Bestrophin-1 (Best1) and bestrophin-2 (Best2) are two members of the bestrophin family of calcium (Ca2+)-activated chloride (Cl−) channels with critical involvement in ocular physiology and direct pathological relevance. The bestrophins are a family of Ca2+-activated anion channels consisting of four members (Best1–4) in mammals. The overall architecture of hBest1 and hBest2 resembles the pentameric assembly previously shown by KpBest, cBest1 and bBest2, and retains the two landmark permeation constrictions, the neck and aperture, in the ion conducting pathway. Ample electrophysiological evidence indicates that the neck and aperture serve as dual Ca2+-dependent channel “gates”, as disrupting either of them partially impairs Ca2+-dependence while disrupting both makes the channel completely Ca2+-independent.

To elucidate the architecture of human bestrophins, we purified WT hBest1 and hBest2 for single-particle cryo-EM analysis in the absence of Ca2+ (EGTA), or after a 30 s spike of 1 μM or 5 mM Ca2+. Under both 1 μM and 5 mM Ca2+ conditions, most of the hBest1/hBest2 particles (~90–95%) were in a Ca2+-bound closed state, which is very similar to the Ca2+-unbound closed state. In both hBest1 and hBest2 structures, the neck is formed by the same set of hydrophobic residues (I76, F80 and F84) as those previously reported in bBest2 and cBest11, underlining a highly conserved neck in bestrophins. On the other hand, the hBest1 aperture exhibits several distinctive features compared to cBest1. Firstly, I205 is the narrowest point (radius 0.9 Å) within the cytosolic region of the ion conducting pathway, similar to I180 in KpBest, whereas the counterpart in cBest1 is V205 (radius 1.3 Å). Secondly, the Q208-N212 pair in hBest1 is connected by a water network in a similar manner to the salt bridge between the K208-E212 pair in h/bBest2, such that Q208 points directly into the central axis of hBest1 (radius 1.8 Å), whereas its counterpart in cBest1 points away from the central axis. This structural divergence is rooted from their different primary sequences: in cBest1, the side chain of Q208 fits in a pocket enabled by G209, whereas a serine at this position in hBest1 (S209) makes a hydrogen bond with Q208, causing the amino group of the Q208 side chain to point directly in towards the central axis. Consistent results were obtained from structural analysis of hBest1 Ca2+-bound datasets, except that residues 346–355 (yellow) and 368–378 (red) were relatively less disordered compared to their counterparts in hBest2, suggesting a stronger binding of this region to the channel periphery in hBest1. Notably, a direct contact between F354 and E300 in hBest1 is disrupted in hBest2 due to an insertion of F at position 353, which also offsets the residue numbers of hBest1 and hBest2 by one within this region.

>[5x]MTITYTSQVANARLGSFSRLLLCWRGSIYKLLYGEFLIFLLCYYIIRFIYRLALTEEQQLMFEKLTLYCDSYIQLIPISFVLGFYVTLVVTRWWNQYENLPWPDRLMSLVSGFVEGKDEQGRLLRRTLIRYANLGNVLILRSVSTAVYKRFPSAQHLVQAGFMTPAEHKQLEKLSLPHNMFWVPWVWFANLSMKAWLGGRIRDPILLQSLLNEMNTLRTQCGHLYAYDWISIPLVYTQVVTVAVYSFFLTCLVGRQFLNPAKAYPGHELDLVVPVFTFLQFFFYVGWLKVAEQLINPFGEDDDDFETNWIVDRNLQVSLLAVDEMHQDLPRMEPDMYWNKPEPQPPYTAASAQFRRASFMGSTFNISLNKEEMEFQPNQEDEEDAHAGIIGRFLGLQSHDHHPPRANSRTKLLWPKRESLLHEGLPKNHKAAKQNVRGQEDNKAWKLKAVDAFKSAPLYQRPGYYSAPQTPLSPTPMFFPLEPSAPSKLHSVTGIDTKDKSLKTVSSGAKKSFELLSESDGALMEHPEVSQVRRKTVEFNLTDMPEIPENHLKEPLEQSPTNIHTTLKDHMDPYWALENRDEAHS>[4x]SRKTYTLTDYLKNTYRLKLYSLRWISDHEYLYKQENNILVFNAEYGNSSVFLENSTFDEFGHSINDYSISPDGQFILLEYNYVKQWRHSYTASYDIYDLNKRQLITEERIPNNTQWVTWSPVGHKLAYVWNNDIYVKIEPNLPSYRITWTGKEDIIYNGITDWVYEEEVFSAYSALWWSPNGTFLAYAQFNDTEVPLIEYSFYSDESLQYPKTVRVPYPKAGAVNPTVKFFVVNTDSLSSVTNATSIQITAPASMLIGDHYLCDVTWATQERISLQWLRRIQNYSVMDICDYDESSGRWNCLVARQHIEMSTTGWVGRFRPSEPHFTLDGNSFYKIISNEEGYRHICYFQIDKKDCTFITKGTWEVIGIEALTSDYLYYISNEYKGMPGGRNLYK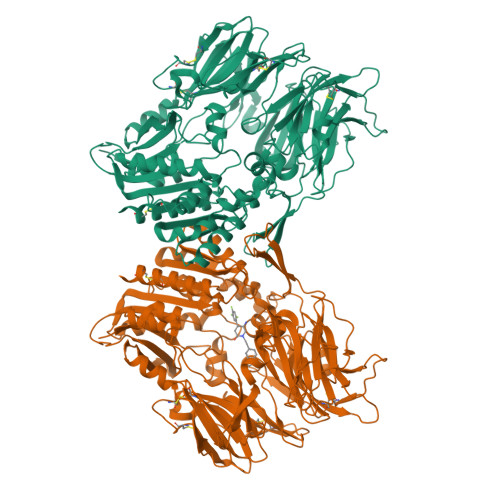IQLSDYTKVTCLSCELNPERCQYYSVSFSKEAKYYQLRCSGPGLPLYTLHSSVNDKGLRVLEDNSALDKMLQNVQMPSKKLDFIILNETKFWYQMILPPHFDKSKKYPLLLDVYAGPCSQKADTVFRLNWATYLASTENIIVASFDGRGSGYQGDKIMHAINRRLGTFEVEDQIEAARQFSKMGFVDNKRIAIWGWSYGGYVTSMVLGSGSGVFKCGIAVAPVSRWEYYDSVYTERYMGLPTPEDNLDHYRNSTVMSRAENFKQVEYLLIHGTADDNVHFQQSAQISKALVDVGVDFQAMWYTDEDHGIASSTAHQHIYTHMSHFIKQCFSLP>MGPVWRKHYITYRINNYTPDMNREDVDYAIRKAFQVWSNVTPLKFSKINTGM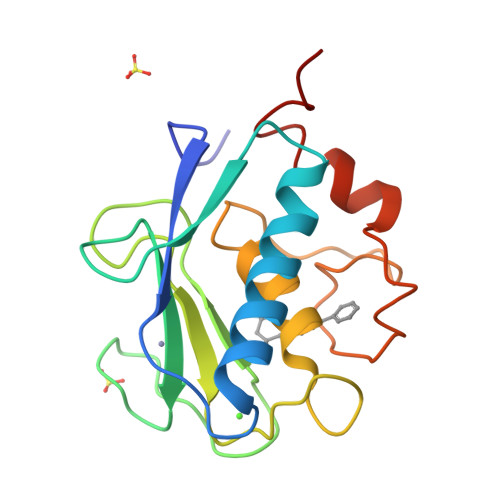ADILVVFARGAHGDFHAFDGKGGILAHAFGPGSGIGGDAHFDEDEFWTTHSGGTNLFLTAVHEIGHSLGLGHSSDPKAVMFPTYKYVDINTFRLSADDIRGIQSLYGDPKEN[4x]> MPISPIETVPVKLKPGMDGPKVKQWPLTEEKIKALVEICTEMEKEGKISKIGPENPYNTPVFAIKKKDSTKWRKLVDFRELNKRTQDFWEVQLGIPHPAGLKQKKSVTVLDVGDAYFSVPLDKDFRKYTAFTIPSINNETPGIRYQYNVLPQGWKGSPAIFQCSMTKILEPFRKQNPDIVIYQYMDDLYVGSDLEIGQHRTKIEELRQHLLRWGFTTPDKKHQKEPPFLWMGYELHPDKWTVQPIVLPEKDSWTVNDIQKLVGKLNWASQIYAGIKVRQLCKLLRGTKALTEVVPLTEEAELELAENREILKEPVHGVYYDPSKDLIAEIQKQGQGQWTYQIYQEPFKNLKTGKYARMKGAHTNDVKQLTEAVQKIATESIVIWGKTPKFKLPIQKETWEAWWTEYWQATWIPEWEFVNTPPLVKLWYQLEKEPIIGAETFYVDGAANRETKLGKAGYVTDRGRQKVVPLTDTTNQKTELQAIHLALQDSGLEVNIVTDSQYALGIIQAQPDKSESELVSQIIEQLIKKEKVYLAWVPAHKGIGGNEQVDGLVSAGIRKVLHHHHHHHHHH;> MPISPIETVPVKLKPGMDGPKVKQWPLTEEKIKALVEICTEMEKEGKISKIGPENPYNTPVFAIKKKDSTKWRKLVDFRELNKRTQDFWEVQLGIPHPAGLKQKKSVTVLDVGDAYFSVPLDKDFRKYTAFTIPSINNETPGIRYQYNVLPQGWKGSPAIFQCSMTKILEPFRKQNPDIVIYQYMDDLYVGSDLEIGQHRTKIEELRQHLLRWGFTTPDK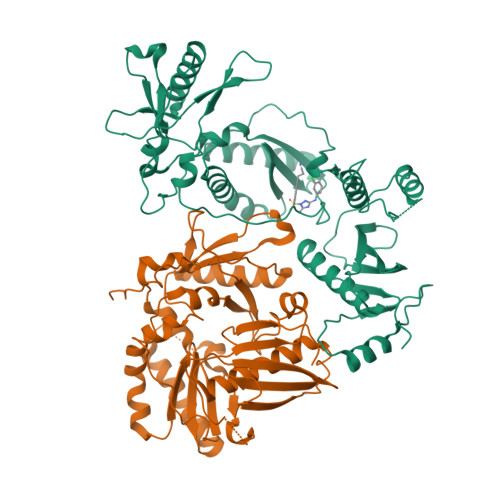KHQKEPPFLWMGYELHPDKWTVQPIVLPEKDSWTVNDIQKLVGKLNWASQIYAGIKVRQLCKLLRGTKALTEVVPLTEEAELELAENREILKEPVHGVYYDPSKDLIAEIQKQGQGQWTYQIYQEPFKNLKTGKYARMKGAHTNDVKQLTEAVQKIATESIVIWGKTPKFKLPIQKETWEAWWTEYWQATWIPEWEFVNTPPLVKLWYQLEKEPIIGAETF>MASMKVAVLPGDGIGPEVTEAALKVLRALDEAEGLGLAYEVFPFGGAAIDAFGEPFPEPTRKGVEEAEAVLLGSVGGPKWDGLPRKIRPETGLLSLRKSQDLFANLRPAKVFPGLERLSPLKEEIARGVDVLIVRELTGGIYFGEPRGMSEAEAWNTERYSKPEVERVARVAFEAARKRRKHVVSVDKANVLEVGEFWRKTVEEVGRGYPDVALEHQYVDAMAMHLVRSPARFDVVVTGNIFGDILSDLASVLPGSLGLLPSASLGRGTPVFEPVHGSAPDIAGKGIANPTAAILSAAMMLEHA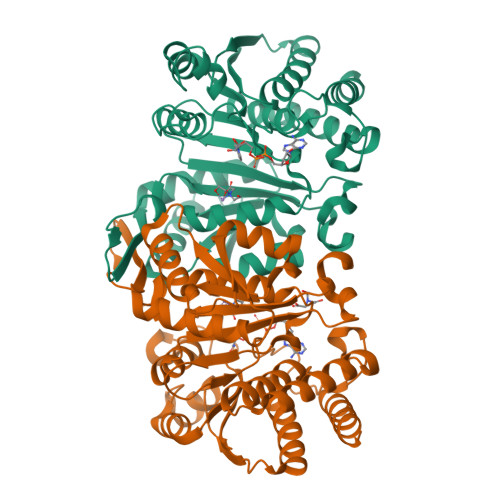FGLVELARKVEDAVAKALLETPPPDLGGSAGTEAFTATVLRHLAAAALEHHHHHH[4x]1-METHYL-1,6-DIHYDROPYRIDIN-3-AMINE | C6 H10 N2 | 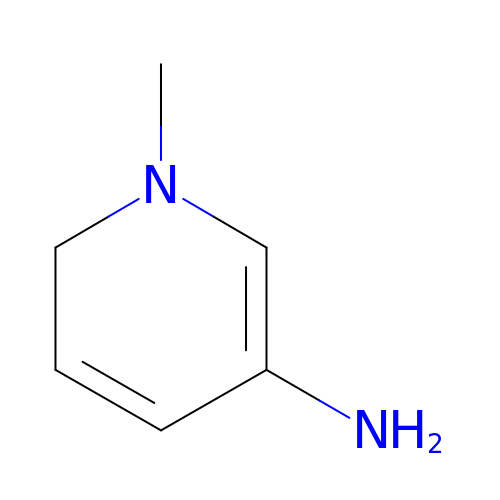NJIDBKRVRJXCLL-UHFFFAOYSA-N> MTTYLEFIQQNEERDGVRFSWNVWPSSRLEATRMVVPVAALFTPLKERPDLPPIQYEPVLCSRTTCRAVLNPLCQVDYRAKLWACNFCYQRNQFPPSYAGISELNQPAELLPQFSSIEYVVLRGPQMPLIFLYVVDTCMEDEDLQALKESMQMSLSLLPPTALVGLITFGRMVQVHELGCEGISKSYVFRGTKDLSAKQLQEMLGLSKVPLTQATRGPQVQQPPPSNRFLQPVQKIDMNLTDLLGELQRDPWPVPQGKRPLRSSGVALSIAVGLLECTFPNTGARIMMFIGGPATQGPGMVVGDELKTPIRSWHDIDKDNAKYVKKGTKHFEALANRAATTGHVIDIYACALDQTGLLEMKCCPNLTGGYMVMGDSFNTSLFKQTFQRVFTKDMHGQFKMGFGGTLEIKTSREIKISGAIGPCVSLNSKGPCVSENEIGTGGTCQWKICGLSPTTTLAIYFEVVNQHNAPIPQGGRGAIQFVTQYQHSSGQRRIRVTTIARNWADAQTQIQNIAASFDQEAAAILMARLAIYRAETEEGPDVLRWLDRQLIRLCQKFGEYHKDDPSSFRFSETFSLYPQFMFHLRRSSFLQVFNNSPDESSYYRHHFMRQDLTQSLIMIQPILYAYSFSGPPEPVLLDSSSILADRILLMDTFFQILIYHGETIAQWRKSGYQDMPEYENFRHLLQAPVDDAQEILHSRFPMPRYIDTEHGGSQARFLLSKVNPSQTHNNMYAWGQESGAPILTDDVSLQVFMDHLKKLAVSSA;> EGLRVVNLLQERNMLPSTPLKPPVPNLHEDIQKLNCNPELFRCTLTSIPQTQALLNKAKLPLGLLLHPFKDLVQLPVVTSSTIVRCRSCRTYINPFVSFLDQRRWKCNLCYRVNDVPEEFLYNPLTRVYGEPHRRPEVQNATIEFMAPSEYMLRPPQPPVYLFVFDVSHNAVETGYLNSVCQSLLDNLDLLPGNTRTKIGFITFDSTIHFYGLQESLSQPQMLIVSDIEDVFIPMPENLLVNLNESKELVQDLLKTLPQMFTKTLETQSALGPALQAAFKLMSPTGGRMSVFQTQLPTLGVGALKPREEPNHRSSAKDIHMTPSTDFYKKLALDCSGQQVAVDLFLLSGQYSDLASLGCISRYSAGSVYYYPSYHHQHNPVQVQKLQKELQRYLTRKIGFEAVMRIRCTKGLSIHTFHGNFFVRSTDLLSLPNVNPDAGYAVQMSVEESLTDTQLVSFQSALLYTSSKGERRIRVHTLCLPVVSTLNDVFLGADVQAISGLLANMAVDRSMTASLSDARDALVNAVIDSLSAYRSSVLSNQQPGLMVPFSLRLFPLFVLALLKQKSFQTGTNARLDERIFAMCQVKNQPLVYLMLTTHPSLYRVDNLSDEGALNISDRTIPQPPILQLSVEKLSRDGAFLMDAGSVLMLWVGKNCTQNFLSQVLGVQNYASIPQPMTDLPELDTPESARIIAFISWLREQRPFFPILYVIADESPMKANFLQNMIEDRTESALSYYEFLLHIQQQVNK;> MVLLTMIARVADGLPLAASMQEDEQSGRDLQQYQSQAKQLFRKLNEQSPTRCTLEAGAMTFHYIIEQGVCYLVLCEAAFPKKLAFAYLEDLHSEFDEQHGKKVPTVSRPYSFIEFDTFIQKTKKLYIDSRARRNLGSINTELQDVQRIMVANIEEVL;> EVTSII

The packaging of cargo transmembrane proteins into COPII-coated vesicles entails a direct interaction between COPII protein and cytoplasmically-oriented ER export signals. About a half dozen export signals have been identified to date, almost all comprising short peptide motifs, all of them binding to the Sec24 subunit of the COPII inner coat. The ΦC export signal was identified in studies of p24-family and ERGIC-53 proteins, and comprises a C-terminal signature of a pair of hydrophobic residues or a single terminal valine residue. The ΦC motif contacts a site on Sec24a that is also the binding site for the LxxLE- and DxE-class export motifs (Miller et al., 2003; Mossessova et al., 2003).

A series of ΦC-signal peptides was synthesized, based on a core sequence of yeast Emp24p, and individual peptides were soaked at high concentrations into two crystal forms of human COPII protein: one comprising Sec23a/Sec24a•Sec22b, the other Sec24c. For all ΦC sequences, we observed clear evidence for peptide binding to a site on Sec24a in the Sec23a/Sec24a•Sec22b crystals, based on the presence of residual electron density that matches the peptide sequence (this binding site is occluded in the Sec24c crystals). (B) Close-up view of the B site on Sec24a with bound ΦC sequence containing the terminal Ile-Ile motif (colored purple) of the S. cerevisiae p24 protein Erv25p. Green contour lines show residual electron density (Fo-Fc synthesis with no phase bias) at 2.6 Å resolution, contoured at 2.6 σ. Electron density is also observable for N-terminal residues of the peptide (residues colored light grey). Thus, specific recognition of the ΦC motif involves the terminal carboxylate group bonding to Arg750 and Arg752 of Sec24a, with the penultimate hydrophobic residue of the motif nestling against Tyr496, and the terminal hydrophobic residue fitting to a pocket of hydrophobic side chains.>[4x]MEEAPLFPGESIKAIVKDVMYICPFMGAVSGTLTVTDFKLYFKNVERDPHFILDVPLGVISRVEKIGAQSHGDNSCGIEIVCKDMRNLRLAYKQEEQSKLGIFENLNKHAFPLSNGQALFAFSYKEKFPINGWKVYDPVSEYKRQGLPNESWKISKINSNYEFCDTYPAIIVVPTSVKDDDLSKVAAFRAKGRVPVLSWIHPESQATITRCSQPLVGPNDKRCKEDEKYLQTIMDANAQSHKLIIFDARQNSVADTNKTKGGGYESESAYPNAELVFLEIHNIHVMRESLRKLKEIVYPSIDEARWLSNVDGTHWLEYIRMLLAGAVRIADKIESGKTSVVVHSSDGWDRTAQLTSLAMLMLDSYYRTIKGFETLVEKEWISFGHRFALRVGHGNDNHADADRSPIFLQFVDCVWQMTRQFPSAFEFNELFLITILDHLYSCLFGTFLCNCEQQRFKEDVYTKTISLWSYINSQLDEFSNPFFVNYENHVLYPVASLSHLELWVNYYVRWNPRMRPQMPIHQNLKELLAVRAELQKRVEGLQREVATRAVSSSSERGSSPSHSATSVHTSV

MTMRs are part of a large group of tyrosine/dual-specificity phosphatase superfamily (PTP/DUSP) members in eukaryotes. Typically, the active MTMRs catalyze the dephosphorylation of phosphatidylinositol 3-monophosphate (PI(3)P) and/or phosphatidylinositol 3,5-bisphosphate (PI(3,5)P2) to produce PI and PI(5)P, respectively. Most MTMRs possess Pleckstrin homology (PH)-GRAM and coiled-coil (CC) domains in addition to the phosphatase (PTP) domain, and some MTMRs contain extra domains, such as differentially expressed in normal and neoplastic cells (DENN), PH, and FYVE domains. In this study, we determined the crystal structure of the PH-GRAM and active PTP domains of human MTMR1 and investigated its substrate specificity through enzymatic and mutagenesis assays.

The MTMR1 structure was determined by molecular replacement using the MTMR2 structure as the search model and refined to 2.07 Å resolution. The refined model included four MTMR1 molecules (A, B, C, and D chains), 652 water molecules, and 6 phosphate ions in the asymmetric unit. The refined MTMR1 monomer structure was composed of 14 β-strands (β1−β14) and 17 α-helices (α1−α17) that formed two individual domains: the PH-GRAM domain (residues 98–205) and the PTP domain (residues 226–605). The PH-GRAM domain, which was originally implicated in protein or lipid binding during membrane-associated processes, exhibited a β-sandwich structure formed by seven β-strands (β1−β7) and one α-helix (α1) that was similar to the MTMR2 structure. The residues of the C(X)5R motif in the active site (Cys438 (here, mutated to Ser438 for crystallization), Ser439, Asp440, Gly441, Trp442, Asp443, and Arg444) were aligned in a loop between β14 and α9. In the MTMR1 and MTMR2 structures, the PH-GRAM domain bound tightly to the large and shallow cleft of the PTP domain formed by residues in and around three helices (α6, α13 and α17) and a loop located between α11 and α12. Among them, one phosphate molecule (D3 phosphate site of PI) was positioned in the deep cleft of the active site pocket and was mainly trapped by its interaction with the main chains of the six residues (Ser(Cys)438, Ser439, Gly441, Trp442, Asp443, and Arg444) from the C(X)5R motif. The second phosphate molecule, which is positioned at the D1 site of PI and only found in two MTMR1 molecules (chains A and B) in the asymmetric unit, interacts with the side chains of Asn351, Ser439, and Arg444. The side chains of Asp440 and Asp443 are positioned away from the active site cavity because of the formation of hydrogen bonds with the side chains of Lys285 and Arg484, respectively, creating sufficient space for the phosphate ion or D3 portion of the substrate. The molecular packing of MTMR1 in the crystal did not show any oligomeric association.> QEHEPIGAQDERLSTLIHQRMQEAKVPALSVSVTIKGVRQRFVYGVADVASQKANTLDTVYELGAMSKAFTGLVVQILIQEGRLRQGDDIITYLPEMRLNYQGKPASLTVADFLYHTSGLPFSTLARLENPMPGSAVAQQLRNENLLFAPGAKFSYASANYDVLGAVIENVTGKTFTEVIAERLTQPLGMSATVAVKGDEIIVNKASGYKLGFGKPVLFHAPLARNHVPAAYIHSTLPDMEIWIDAWLHRKALPATLREAMSNSWRGNSDVPLAADNRILYASGWFIDQNQGPYISHGGQNPNFSSCIALRPDQQIGIVALANMNSNLILQLCADIDNYLRIGKYADGAGDAITATDTLFVYLTLLLCFWGAVVVVRGAFRVYRATAHGPGKQQRLRLRVRDYIIALAVPGLVAAMLYVAPGIMSPGLDWRFILVWGPSSVLAIPFGMILLAFVLTLNHQIKRILLHNKEWDDEHHHHHH

Colibactin, a DNA cross-linking agent produced by gut bacteria, is implicated in colorectal cancer. Its biosynthesis uses a prodrug resistance mechanism: a non-toxic precursor assembled in the cytoplasm is activated after export to the periplasm. Although the transmembrane domain is required for colibactin activation, its role in catalysis is unclear.

To better understand the role of the ClbP TMD in enzymatic function, we determined the crystal structure of full-length ClbP embedded in a lipid mesophase. Seeking structures in the presence of substrate analogs, we initially focused on the catalytically inactive S95A variant. Early S95A crystals yielded electron density maps that clearly showed the position of individual transmembrane helices, although their resolution was insufficient to assign the registry or helix connectivity pattern. To overcome this challenge, we mutated non-conserved TMD positions to methionine—L454M and I478M—and used anomalous diffraction data from selenomethionine-substituted crystals to locate these sequence markers in electron density maps. We obtained two high-resolution structures of S95A-L454M-I478M: selenomethionine-substituted ClbP and methionine-containing ClbP bound to a product analog. The resulting high-quality maps allowed us to fully model the TMD helices and unambiguously assign their registry. The two structures are nearly identical (root mean squared deviation (RMSD) = 0.15 Å over the Cα carbons of residues 38–414 and 431–491), except for the extent to which the TMD’s intracellular loops are modeled; we base our analysis below on the higher-resolution product-bound structure. We initially crystallized S95A-L454M-I478M in a precipitant solution supplemented with compound 1 and obtained a 2.7-Å structure that suggested that monoolein, the crystallization lipid, was bound at the active site. In our model, the headgroup of monoolein forms polar interactions with active site residues S188 and H257. The chemical similarity to myristoyl-d-asparagine suggests that monoolein acts as a substrate mimic.>MIFTLRPYQQEAVDATLNHFRRHKTPAVIVLPTGAGKSLVIAELARLARGRVLVLAHVKELVAQNHAKYQALGLEADIFAAGLKRKESHGKVVFGSVQSVARNLDAFQGEFSLLIVDECHRIGDDEESQYQQILTHLTKVNPHLRLLGLTATPFRLGKGWIYQFHYHGMVRGDEKALFRDCIYELPLRYMIKHGYLTPPERLDMPVVQYDFSRLQAQSNGLFSEADLNRELKKQQRITPHIISQIMEFAATRKGVMIFAATVEHAKEIVGLLPAEDAALITGDTPGAERDVLIENFKAQRFRYLVNVAVLTTGFDAPHVDLIAILRPTESVSLYQQIVGRGLRLAPGKTDCLILDYAGNPHDLYAPEVGTPKGKSDNVPVQVFCPACGFANTFWGKTTADGTLIEHFGRRCQGWFEDDDGHREQCDFRFRFKNCPQCNAENDIAARRCRECDTVLVDPDDMLKAALRLKDALVLRCSGMSLQHGHDEKGEWLKITYYDEDGADVSERFRLQTPAQRTAFEQLFIRPHTRTPGIPLRWITAADILAQQALLRHPDFVVARMKGQYWQVREKVFDYEGRFRLAHELRG[2x]

RadD, a member of the SF2 family, is a recently discovered DNA repair protein involved in the repair of DSBs after radiation or chemical damage. RadD is classified into the helicase superfamily (SF) 2, which contains all seven conserved motifs of SF2 and a small homology sequence outside of these motifs. Here, we reported the crystal structures of E. coli RadD/ATPγS and RadD/ATP at 3.0 Å and 2.7 Å, respectively. An ATPγS or ADP molecule was buried between RD1 and RD2.

RadD/ATP crystals were obtained by incubating and co-crystallizing 5 mg/mL RadD and 5 mM ATP with 5 mM Mg2+. The electron density of the structure showed only the density of the ADP molecule and no density of γ-phosphate, indicating that ATP was hydrolyzed into ADP during crystallization. However, in the structure of the RadD/ATP complex, an ADP molecule was at the same position as ATPγS. However, in our structure of RadD/ATP, Ser38 solidly interacted with the Mg2+ ion, Asp117 was away from the Mg2+ ion, and Lys37 was in the middle of Asp117 and γ-phosphate of ATP at a distance of 3.2 Å and 3.5 Å, respectively. The side chain of Lys37 and Asp117 moved away from the γ-phosphate of ATP in the structure of RadD/ATP compared with the apo-RadD. Lys37 is located between the γ-phosphate of ATP and Asp117, which are on the same line and form an equilibrium state by the electrostatic attraction. The side chain of Lys37 shifts away due to the exit of the ADP molecule, and Asp117 will correspondingly move back to its prepolarized attacking water configuration. Crystals of RadD/ATP were obtained by incubating 5 mg/mL RadD and 5 mM ATP for 30 min at 20 °C, and grown under the same conditions as RadD/ATPγS, except that Mg2+ ion was added to the solution (500 mM NaCl, 5 mM MgCl2, 18% (w/v) PEG3350).> GSHMDSTTIQQNKDTLSQIVVFPTGNYDKNEANAMVNRLANIDGKYLNALKQNNLKIKLLSGKLTDEKEYAYLKGVVPKGWEGTGKTWDDVPGLGGSTVALR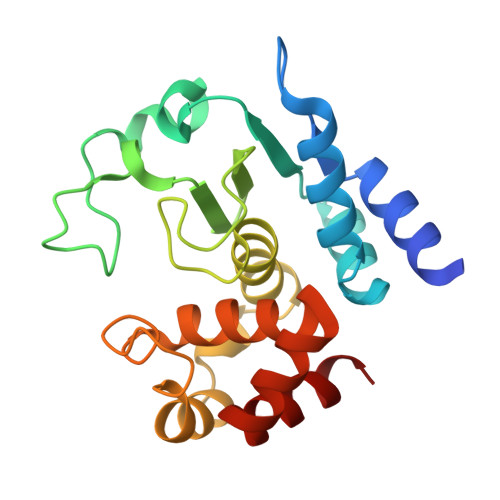IGFSNKGKGHDAINLELHATAHAIDHIVLNDISKSAQFKQIFAKEGRSLGNVNYLGVYPEEFFAESFAYYYLNQDTNSKLKSACPQTYSFLQNLAK> MKLIWSEESWDDYLYWQETDKRIVKKINELIKDTRRTPFEGKGKP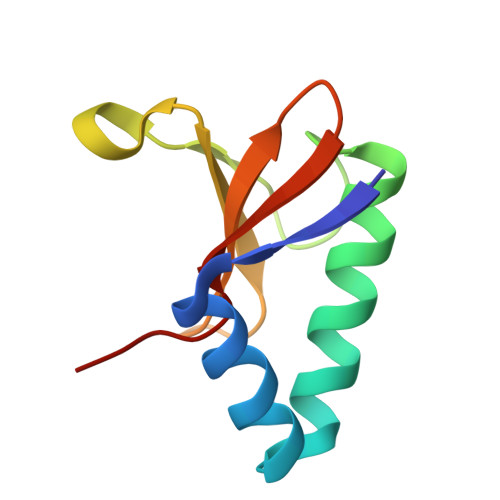EPLKHNLSGFWSRRITEEHRLVYAVTDDSLLIAACRYHY>GG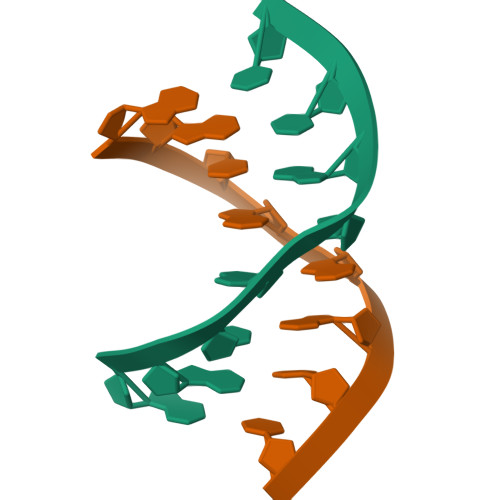CGAGCC[5x]> MGRQWALEDFEIGRPLGKGKFGNVYLAREKQSKFILALKVLFKAQLEKAGVEHQLRREVEIQSHLRHPNILRLYGYFHDATRVYLILEYAPLGTVYRELQKLSKFDEQRTATYITELANALSYCHSKRVIHRDIKPENLLLGSAGELKIADFGWSVHAPSSRRTTLCGTLDYLPPEMIEGRMHDEKVDLWSLGVLC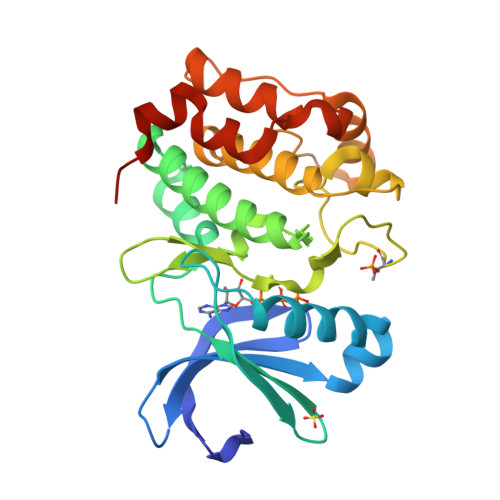YEFLVGKPPFEANTYQETYKRISRVEFTFPDFVTEGARDLISRLLKHNPSQRPMLREVLEHPWITANSSKPHHHHHH>[6x]GPMDFSINPPQRIVFVGLGTIAQSFLPLLSKVHDLSTLEIYAIDPKTPPLIEYFANSFGLKFINS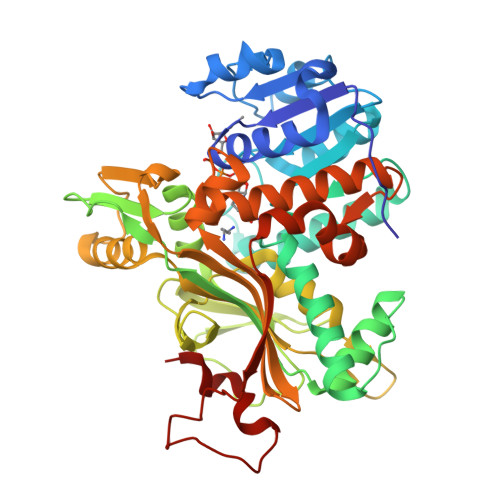AIDQINYRDILVPILGEGTVLINLSTDVSSLALIELCRSAGALYLDTCIEPWKGGYDDPTIPLHKRTNYHLREQMLSLKKRLGSGVTALVAHGANPGLVSHFVKRALLDLAEEILGDCKKPSNKEQWAILSQRLGVKVIHVAEYDSQISQKSRERGEFVNTWSVHGFISESQQPAELGWGSHERSLPTDASMHTDGCGAAIYIEKPGASVRVKTWTPFNGPSLGYLVTHHEAISIADFLTLRTADETYRPTVHYAYRPSDEAILSVHEWFGNDCMTPEKTKVLRPGDILSGSDYLGVLLMGHEKSSYWYGSILSIEKAKELATLNTATTLQVAAGVLSGYLWILSHPSAGIIEAEDMDHEVALSYISQYLGELKGVYSDWNPTKNNPGTFSAIDSDSPWLFSNFVL3-[3-(TERT-BUTYLTHIO)-1-(4-CHLOROBENZYL)-5-(QUINOLIN-2-YLMETHOXY)-1H-INDOL-2-YL]-2,2-DIMETHYLPROPANOIC ACID | C34 H35 Cl 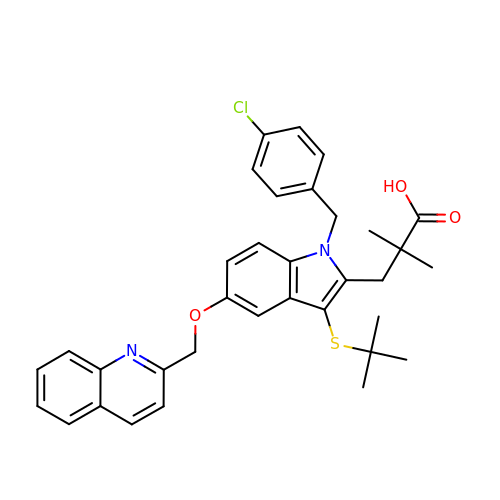N2 O3 S | NZOONKHCNQFYCI-UHFFFAOYSA-N>[2x]ACDYTCGSNCYSSSDVSTAQAAGYKLHEDGETVGSNSYPKKYNNYEGFDFSVSS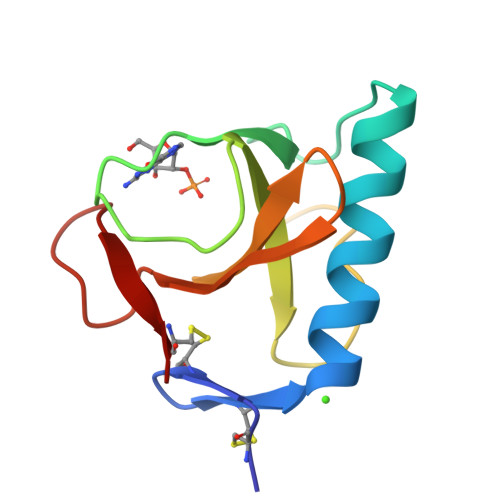PYYEWPILSSGDVYSGGSPGADRVVFNENNQLAGVITHTGASGNNFVECT> MSRTTPPHPAEIVAHLQPEIWNKVNRLLVRKAISEYAHEWLLEPQRLGPGETPGFERFRLTLADGAQYDFDAQVMAMRHWRIPPESIVKTVAGVPAPLDALQFVIEIRDKLGLPVDRLPIYMDEITSTLHGSAYKHGRTTLGAAALARADYQTIETSMIEGHPSFVANNGRLGFDAEDYHGYAPEAATPVRLMWLAVHKDNAHFSCLSDMDYDSLMSEELGESAVTDFAARLREQGLHPADYYFMPAHPWQWFNKLSLAFAPYVAQRKIVCLGYGEEQYLAQQSIRTFFNISRPGKRYVKTSLSILNMGFMRGLSPYYMAGTPAINEYIHDLISADPWLRANGFRILREVASMGFRNYYYEAAIDTDTPYKKMFSAL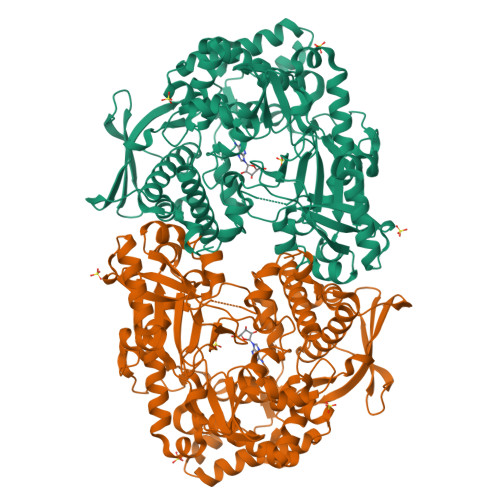WRENPLTLIAPGQNLMTMAALLHVDPQGRALLPELIQASGLDAGTWLERYVDAYLTPLIHCFYAHDLVFMPHGENVILVIQDGVPVRAFMKDIAEESSILNPQVRLPQAAQRLAADVPEAYKLLTIFVDVFEGYFRHLTQILVETELMPEHDFWRLVAGRIAAYQQAHPQRLDKYRRYDLFAPDMIHSCLNRLQLANNLQMVNLADPIGSFQMAPNLPNPIACFRPSWLGSGEALQTLTAA>SPRMDDHGLKEICLDHLYRGCQ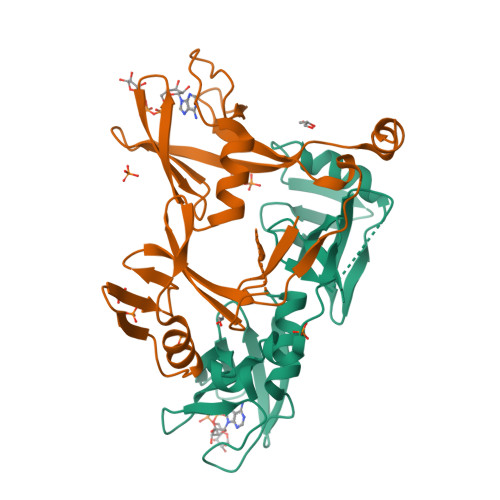QVNCNKNHFHLPYRWQLFILPTWMDFQDMEYIERAYCDPQIEIIVIEKHRINFKKMTCDSYPIRRLSTPSFVEKTLNSVFTTKWLWYWRNELNEYTQYGHESPSHTSSEINSAYLESFFHSCPRGVLQFHAGSQNYELSFQGMIQTNIASKTQRHVVRRPVFVSSKDVEQKRRGPD[2x]> SGAYDVTWDSVAWKNSAAKPWLGSMPLGNGDLGLNVWVEENGDLVFLIGKTDAWSENGELLKLGRVRLHLAASPLVAKSFRQVLKPEEGAVEVYSPADAPRPLYRVWVDANHPVAHVEVRTASGKATGAQADLELWRNEPREVRRVKGRERDNVEFNDGFRELRDTPGSLVTVDPDTVLPAKPGGDRIAWCHHNGRSLYPALLANQHLESLLPKYPDPLLNRTFGAVLEGPGFVASGDRTLKLMKESA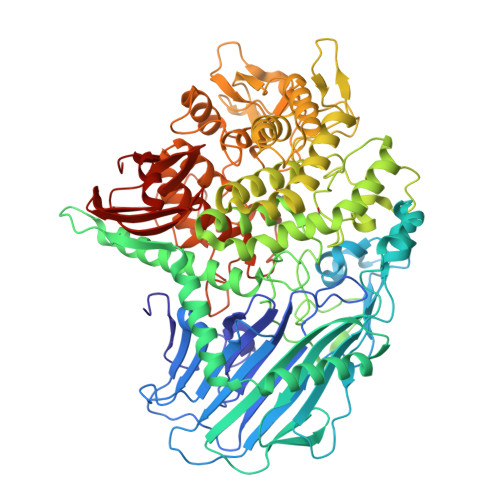AFRLDLYALATTAPDVEAWADDAGVLADTLSGLDIEAARLAHRNWWRAFWGRSWIVVDGNDLPGGDPTDGEMARAVTQSYAMQRWMTAGSGRSVAAMPIPFNGAIFTVGKETPKEKYDPAKGDTGNPDFRTGGGNIPFQNTRHIYWPMLASGDYDLMRPFFRRYRENLALLTERTRLYDKHAGAAFPETGFFWGLPNDADFGIGNKEAVLQNLAIRYEIQGGLELTAMMLDYYDATQDTDFLVNTLLPLADGVAAYYDQHWQRGGDGKIVFSPAQSLTTYQSPSGKDVVNPLPDIAGLMAVLPRLIALPPGTATAAQRTAWKKTLADLPPLPRGKTGTGRNNTPDKVPIPSTTQKDDGAPILLPAQVYGTEKNVENPEEYAIFPYRLFGVGLPEIDLGLNTFRARNFTDSTGWAWDGIVAACLGLSDDAKREAIRNFAEDRNPDTGHGPNYPGLSAFSREARFKWFWKPGPSSGPGNGTEPALDNGGVGQSILQSMLLQQRGEKIVLFPAWPKEWNVSFKLHAARNTTVEGVLKNGKLERLTVTPPERRGDVIVREAQ>SRAPAPATPHAPDHSPAPNSPTLTRPPEGPKFPRVKNWELGSITYDTLCAQSQQDGPCTPRRCLGSLMLPRKLQTRPSPGPPPAEQLLSQARDFINQYYSSIKRSGSQAHEERLQEVEAEVASTGTYHLRESELVFGAKQAWRNAPRCVGRIQWGKLQVFDARDCSSAQEMFTYICNHIKYATNRGNLRSAITVFPQRAPGRGDFRIWNSQLVRYAGYRQQDGSVRGDPANVEITELCIQHGWTPGNGRFDVLPLLLQAPDEAPELFVLPPELVLEVPLEHPTLEWFAALGLRWYALPAVSNMLLEIGGLEFSAAPFSGWYMSTEIGTRDLCDPHRYNILEDVAVCMDLDTRTTSSLWKDKAAVEINLAVLHSFQLAKVTIVDHHAATVSFMKHLDNEQ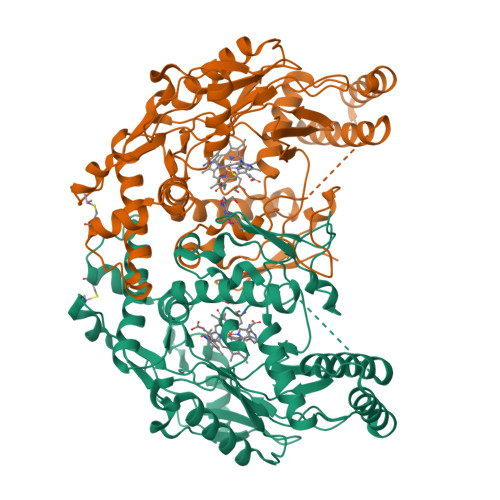KARGGCPADWAWIVPPISGSLTPVFHQEMVNYILSPAFRYQPDPW[2x]>VIPVASPDPALVNNPVVAATEPSVVKIRSLAPRCQKVLEGTGFVISPDRVMTNAHVVAGSNNVTVYAGDKPFEATVVSYDPSVDVAILAVPHLPPPPLVFAAEPAKTGADVVVLGYPGGGNFTATPARIREAIRLSGPDIYGDPEPVTRDVYTIRADVE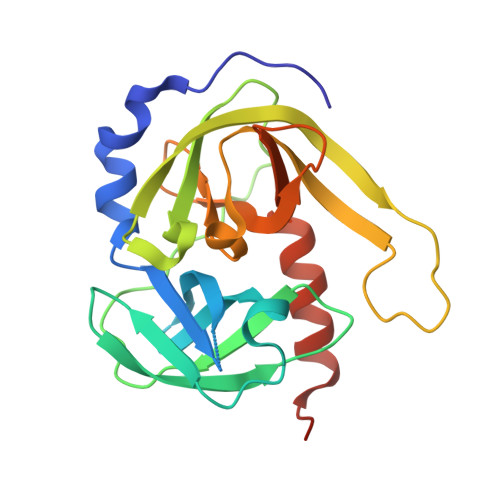QGDAGGPLIDLNGQVLGVVFGAAIDDAETGFVLTAGEVAGQLAKIGATQPVGTGACVS[2x]> MLNQELELSLNMAFARAREHRHEFMTVEHLLLALLS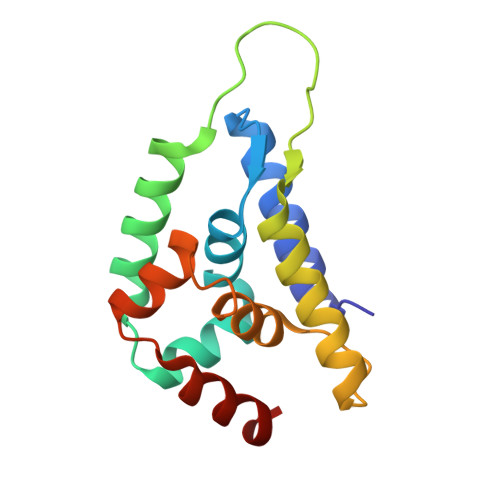NPSAREALEACSVDLVALRQELEAFIEQTTPVLPASEEERDTQPTLSFQRVLQRAVFHVQSSGRNEVTGANVLVAIFSEQESQAAYLLRKHEVSRLDVVNFISHGTR Here, we focus on the identification and characterization of proteins selectively secreted by the first larval stages of T. suis. We screened a set of n = 6 recombinant larval proteins for immunomodulatory properties and identified an enzymatically active T. suis chitinase that interfered with recruitment of immune cells and inflammatory reactions in a murine model of allergic airway disease. While our in vitro data suggest no direct immunomodulatory effects on, e.g., DC function or T cell activation, we observed disease amelioration to be associated with suppression of eosinophil recruitment into the lung and increased numbers of alternatively activated RELMα+ lung macrophages. Since mammalian host chitinases, both true chitinases with enzymatic activity (AMCase and chitotriosidase) and chitinase-like protein (CLP) molecules which can bind to chitin but lack enzymatic activity, are implicated as either mediators or biomarkers involved in airway inflammation and fibrosis, disease amelioration by treating with a worm chitinase was rather surprising.

X-ray crystallography revealed the structure of the nematode enzyme to be highly similar to the host's own chitinases. The three-dimensional structure of the T. suis chitinase as determined by high-resolution X-ray crystallography revealed high similarities to mouse acidic mammalian chitinase (AMCase) but a unique ability of T. suis chitinase to form dimers. Our data indicate that the structural similarities between the parasite and host chitinase contribute to the disease-ameliorating effect of the helminth-derived chitinase on allergic lung inflammation. Our findings further reveal that T. suis chitinase treatment of allergic mice not only inhibited host AMCase expression on mRNA level but also interfered with host chitinase activity in the BAL fluid, suggesting an alternative mechanism that might involve the high degree of structural similarity between host and nematode chitinases.

>[6x]AAESGARSVCNTVRRRSAGMLRKDSQDASDEKYVRGCYFTNWAQYRPGNGKYNPEHYQANLCEYIFYAFAKLNDDFTVDQFEWNDIDVLYPGVMKQKSSQPDLKVLLSLGGWNAGTATFKKMAATYSNRAKFISSLVSFLQQNKFDGFDLDWEYPESSDKENYLLLCQEILAKFEEVAKCTSTSRLLFTAAVSANPKTVDAGYDVPALAKVLDFVNLMCYDFHGAWETQTGINSPLYSRKEDSSEFKMWNVEQSSKYWSDKGMPKKQIIIGLPTYGRGWTLSDASKTDIGAPAQGSSTATEYLREAGVISYYEVCQKLSSGAKRVWDDESKTPYLVQGNQWFSYDDVESMKAKINWIKQENYGGAFVWTLDYDDFLGSFCTEHNGKKYPLISLMQEILGGGYVPPSTESTTSQVTTTPSTTTSTTSPAGAFQCPSDGLFPDPESCSNFYQCAGGTAYKMKCPTGLMFNPKTSTCDYPSNVDCQEKTITTHHHHHH Plexins are a large group of type I transmembrane proteins that serve as the major receptors for semaphorins. The plexin cytoplasmic region contains a juxtamembrane segment, a RhoGTPase binding domain (RBD) and a GTPase activating protein (GAP) domain. Instead it is active specifically to the Ras homolog Rap, and this RapGAP activity is critical for plexin signaling. Semaphorin binding to the plexin extracellular region induces formation of the active dimer of the cytoplasmic region, which triggers its GAP activity to inactivate Rap through the non-canonical catalytic mechanism for signal transduction.

We therefore removed the linker and directly fused the coiled-coil with the juxtamembrane helix (the N-terminal helix in the juxtamembrane segment) of plexincyto. In the CC(a)PlexinC1cyto structure, the two plexin monomers in the asymmetric unit form a symmetric side-by-side dimer. The two juxtamembrane helices are oriented approximately in parallel, extending well beyond the main body of the proteins and integrating into the C-termini of the coiled-coil moiety. The dimer interface is formed by the juxtamembrane helix and one side of the GAP domain, burying a total of ∼3200 Å2 surface area. The center of the dimer interface is a 4-helix bundle structure comprised of the C-terminal portion of the juxtamembrane helix (residues 567–584) and the N-terminal portion of helix 11 in the GAP domain (residues 929–943) from each monomer. The core of the 4-helix bundle is dominated by hydrophobic interactions, involving residues Ile571, Ile575, Phe579 and Leu582 from the juxtamembrane helix and Met933, Ile936 and Leu939 from helix 11. A loop-helix segment (residues 1038–1058) between helix 15 and 17 in the GAP domain of each monomer wraps around the C-terminal portion of the 4-helix bundle. In the active dimer structure, the last two turns in the juxtamembrane helix (residues 585–591, corresponding to residues 1282–1288 in mouse PlexinA3) convert to an extended loop. In contrast, the activation segment in the active dimer adopts an open conformation and shifts away from the GAP active site. Therefore, a major mechanism in the dimerization-induced activation of plexin appears to be the outward shift of the activation segment, which opens the otherwise obstructed active site to allow Rap binding and catalysis of GTP hydrolysis.

>GGSVKQLEDKVEELLSKNAHLENEVARLKKLQKQMSKKMNDQLELMESNIRRDIRQGFVDLQTEKSDLIDNVGAIPFLDYKHFASRIFFPEAGTLTAVMIRDIGEDSEQTTVDEKCLAFAELIRDKQFLSCFVHALEEQKNFSIKDKCTVASLLTLALHGDLLYLTEIMEDLLQSLMDQSSNANPKLLLRRTESIVEKLLTNWMSICLYGFLRESVGQPLFLLVSALTQQISKGPVDSVTEKALYTLSEDWLLCQAQDFEPLKLKVVFAVGTGEEISESLEVIALTCDTIQQVKEKILQTFQRKFGFRYTQQIRDIEIEYEKEGKFVMLQEVDDTSEIRGHVTMLNTLKHYQVGDGACIKVITPKIHAPLKTQNSVKDDKNFSIKYFHLVDPDIDTDLSNHPEKKALKIKEMYLIKLLSTKVAVHSFVENLFKSIWGLPNNKAPLAVKYFFDFLDEQAERKKITDPDVLHIWKTNSLPLRFWVNILKNPDFVFSDMEKSPHLDGCLSVIAQAFMDSFSLTDTHLDKHSPTNKLLYGKDIPQYKQEVKSYYKLVKDQTSISSQELKTFLQEESKKHQNEFNESAALRELYKYMQRYFTEIFQKLEQTDAPSNLKENMHRVKELFDNMKRSGWN[2x]> RPESELIRQSWRVVSRSPLEHGTVLFARLFALEPSLLPLFQYNGRQFSSPEDSLSSPEFLDHIRKVMLVIDAAVTNVEDLSSLEEYLTSLGRKHRAVGVRLSSWSTVGESLLYMLEKSLGPDFTPATRTAWSRLYGAVVQAMSRGWDGE

To investigate the correlation between mechanical properties and functional efficiency in proteins, we selected neuroglobin (Ngb), a hexacoordinated heme protein, which is expressed in the neurons of vertebrates and is involved in neuroprotection in hypoxic conditions and protects brain from stroke. Ngb folds like all globins with a bundle of eight helices termed A to H, and a heme hexacoordinated in both ferric and ferrous forms by the imidazole side chain of the distal and proximal histidines (His 64 and His 96 respectively). The structures of human and murine Ngb present a large internal cavity behind the heme, that is connected to the surface through a tunnel, forming a pathway toward the heme for gaseous ligands (O2, CO, NO). Like many recently discovered globins, Ngb is characterized by endogenous heme iron hexacoordination in the absence of external ligands.

MPa - The F106W mutant crystal also seems to be more sensitive to pressure than the WT, but more resilient than the V101F mutant. There are no major differences between F106W HP-280 and F106W HP-310. In particular, the tunnel disappears already at 280 MPa and site I disappears at 310 MPa, while site II remains insensitive to pressure (data not shown). The protein mean B-factors are considerably raised by pressure, which could explain why this mutant is more sensitive to pressure than WT Ngb. The residues whose B-factors present a relevant increase with pressure (more than 15 Å2) are mostly located at the back of the protein, while the residues whose B-factors are moderately increased by pressure (less than 5 Å2) are mainly located close to the heme. The effect of pressure seems to be the opposite of what was previously observed in WT Ngb under pressure. In this mutant, the mechanical nucleus still coincides with the hinge region, but the whole protein behaves in a reverse way compared to WT-Ngb, with the zone close to the heme stabilized by pressure and the zone at the back of the protein destabilized by pressure.>[2x]MTKKRVALIFGGNSSEHDVSKRSAQNFYNAIEATGKYEIIVFAIAQNGFFLDTESSKKILALEDEQPIVDAFMKTVDASDPLARIHALKSAGDFDIFFPVVHGNLGEDGTLQGLFKLLDKPYVGAPLRGHAVSFDKALTKELLTVNGIRNTKYIVVDPESANNWSWDKIVAELGNIVFVKAANQGSSVGISRVTNAEEYTEALSDSFQYDYKVLIEEAVNGARELEVGVIGNDQPLVS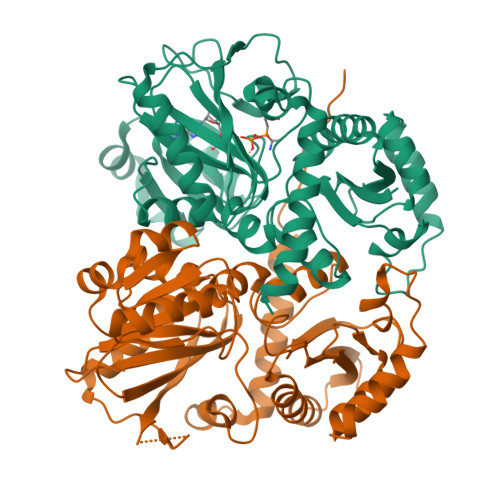EIGAHTVPNQGSGDGWYDYNNKFVDNSAVHFQIPAQLSPEVTKEVKQMALDAYKVLNLRGEARMDFLLDENNVPYLGEPNTLPGFTNMSLFKRLWDYSDINNAKLVDMLIDYGFEDFAQNKKLSYSFVSLGEEKIGKFN> MNEDMGVIVRTNARALIPFIGIFGAYIVTHGHL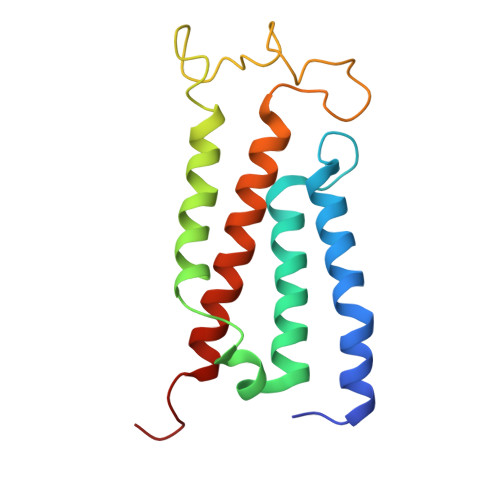TPGGGFQGGATIAGAGVLFLIAFGVKAAKEKINKNLYSALEGLGGLVFLGAAMLGLSVAFFYNILWHEGPIFNSSPGTLLSAGFLPIMNLGVGLKVFTGLVSALFALSVFRRWKS> GSGSGTPAPDAINDLLRSVDSQEVRDYCQKKGWIVIH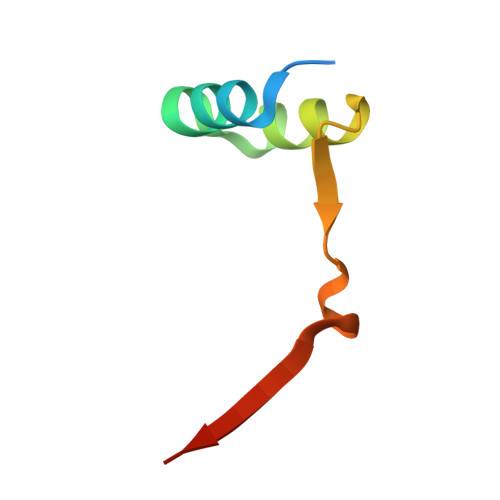PSNELVVEKHISR>[2x]MQEAARRASLRKEHTPTNEKFGDLSKQDSLGERASSKLTLDDELYDILYAFGETDAFINKGDKQRETDEDGNPLTRQALLERIRQKKEVIGKLRCQAWSMTRKRRTLKLAQKYLEQHESKVSRSHLYMEEMRKRARLMKRSFSNFKTYLIPWESKIKRIESHFGSVVSSYFTFLRWIVFVNIMITLIALVFVVLPETLADSVANEGRFNRTKTRK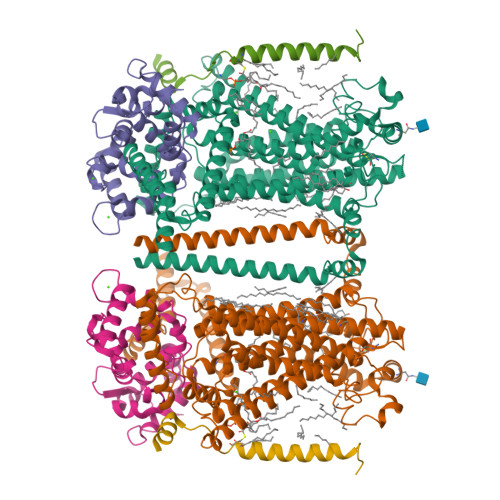QIPANERVHADELAVVWHYDGYLRYSPLFYGYYSDDPFLGNKIKYALPLAYFMVTLTIFAYSFFAILRKMAANARMSKLSGSKAEQYIFNWKLFTGWDYTIGNSETASNTVMAVVIKLRESIADIKKDAHGKFRLLQFSLRVFANIIICAMLGFSIYCIIFAVQKSQVQDDGNLFTKNQVPSVVSTITHVFPMIFDLIGKMENYHPRTALRAHLGRVLILYTVNYITLIFALFEKMTALRDRVNSTSTSSSHRTKRQQGGWNPNMQRPPPYASRAEVRQMSDFLAANTRRFQTVSQRTTRSVTTPFTVAPQFGPFNVNNPNAVFHNGTHSTSFESQILGPKALPIFTPPPRKYPGFTPGNVGQQFGGPDFPRNQVYTKSTPLPRVRTKPPWVYTTTHPPLVQNRAMTTTMSKSAKKGNSKNLDDDILLSNETIQMSEAALRRNHDGHNNDICWETIIGQEIVKLVTMDLIFTILSILVIDLFRGLWIKYCSSWWCWDIETTFPEYGEFKVAENVLHIINNQGMIWLGLFFAPLLPAINNIKLIILMYIRGWAVMTCNVPAREIFRASRSSNFYLGILLIWLLLCTLPVGFVIASMSPSRSCGPFARYQHFYTVVTREIEKRVDQTVLSYIRHIASPGVVIPIILFLILIIYFLFSLVRGLREANTDLQAQLVHERTEEKKKIFELAGGKKNKFEKDRDKKRSNDYIPLIEQRRREPWRQYHEMEADHALASDSSEESDINEDEDDERQPLTAYPLRAIETPPETLQVTAFHPSLGSLIENREMEDEESASGDQLPMIHKSVSFQGPSHMQMRQSISTESCSQISRSAIQVATPEEIRALLRPYLEAKYGIPYQHGIKSFPIDVHTPPNNTPSRRSSKYNSFVSLYEHTRDDHKNFVASTIKETDEDPGKSDKKQTSSKDVAPDFMPWPSADEARALREKMKSKTPLMLTKTTVEEKPKGGKSSESEFRPPVPIHRKYNIQTTEEENEEEETDSAPESSKKRFRISVSPTKTIAPASASRAQHKIVSQASSSSSIPHGRQPDPNKKASLVLPPLRAPRVQFDEDDSPRQID;>[2x]MGNNASSLSELNLFSKGGVFTREQLDEYQDCTFFTRKDIIRLYKRFYALNPHKVPTNMQGNRPAITTLTFEEVEKMPELKENPFKRRICEVFSEDGRGNLSFDDFLDMFSVFSEMAPLQLKLKYAFRIYDYDGDELLGHDDLSKMIRSLTRDELSDVEVEFIIERIIEEADLDGDSSINFAEFEHVVSRSPDFIRTFHIRI;>MPSGNEEINHLSALDQFVAPGLRLWMLIALVGGVLLIMIVIVCCFMRIRIPRTKRQIDLIAAKRKLRKSTKNSAEANAHNDERAQAIVMNSMPSGGGGGAPSTSSSRHTGSRIQSQV[2x]The first step of this process is the transport of sialic acid to the cytoplasm, which often takes place using a tripartite ATP-independent transport system consisting of a periplasmic binding protein and a membrane transporter. In this paper, the structural characterization of periplasmic binding proteins from the pathogenic bacteria Fusobacterium nucleatum, Pasteurella multocida and Vibrio cholerae and their thermodynamic characterization are reported. The structure and the thermodynamics of the binding of sugars suggest that all of these proteins have a very well conserved binding pocket and similar binding affinities. While the C1 carboxylate has been identified as the primary binding site, a second conserved hydrogen-bonding network is involved in the initiation and stabilization of the conformational states.

Vc-SiaP was crystallized without Neu5Ac and we determined its structure to 1.45 Å resolution. These crystals belonged to space group I222. The structure was refined to an R factor of 0.18 and a free R factor of 0.22. However, the r.m.s. deviation between the open form of the Vc-SiaP structure and the open form of the Hi-SiaP structure was about 0.9 Å. Interestingly, a Co atom mediates the inter-protein contact in the crystal lattice. Given that there was no cobalt in our buffers, we propose that this came from the TALON column used in purification. This cobalt appeared to be ligated by three His residues from the C-terminal end of the six-His tag and Glu261 from a neighbouring molecule. Interestingly, the binding affinity of Vc-SiaP is 309 nM, i.e. ten times weaker than those of Fn-SiaP and Pm-SiaP. The structural features that might contribute to the low binding affinity of Vc-SiaP remain unclear.

> ATTLKMGMQASVGSVEYNSAKMLADTLEEMSQGEIKLALYPSAQLGDDRAMLQQLTLGDLDITYAEFGRMGLWIPRAEAVMLPYVAKDFDHLRRMFESDFGQGVRDEMLQKFNWRALDTWYNGTRETTSNRPLNSIEDFKGLKLRVPNAKQNLNYAKLSGASPTPMSFSEVYLALQTNAVDGQENPLPTIKTMKFYEVQKNLAMTHHIVNDQMVIISESTWQKLSDTDKDIIQKAVQKVGDAHTQTVKTQEAELVSFFKSEGINVTYPDLEPFREAMQPLYKEFDSNIGQPIVSKLAAMLQHHHHHH1,3-BIS{4-[(1E)-N-(4,5-DIHYDRO-1H-IMIDAZOL-2-YL)ETHANEHYDRAZONOYL]PHENYL}UREA | C23 H28 N10 O | 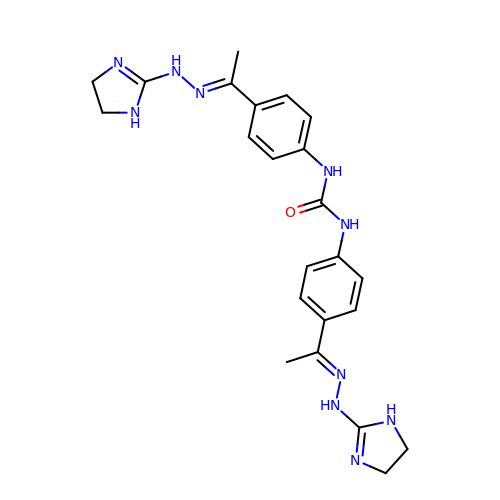IGZOGYCMSGAQFP-KUGLDEIXSA-N> LSSKYSRNT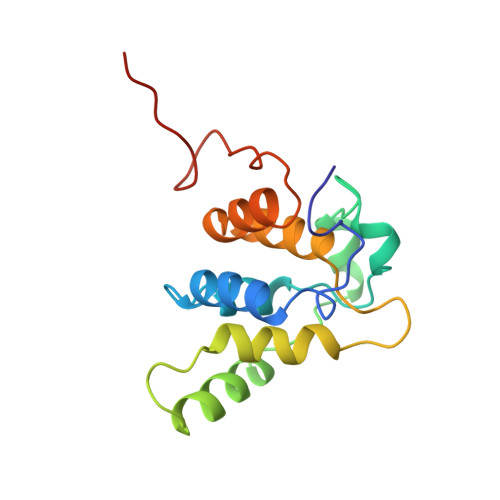ELRRVEDNDIYRLAKILDENSCWRKLMSIIPKGMDVQACSGAGCLNFPAEIKKGFKYTAQDVFQIDEAANRLPPDQSKSQMMIDEWKTSGKLNERPTVGVLLQLLVQAELFSAADFVALDFLNESTPARPVDGPGALISLELLE> MSFPGWGPYPPVERDETSAITYSSKLHGSVTVRDPYSQLEVPFEDSEETKAFVHSQRKFARTYLDENPDREAWLETLKKSWNYRRFSALKPESDGHYYFEYNDGLQSQLSLYRVRMGEEDTVLTESGPGGELFFNPNLLSLDGNAALTGFVMSP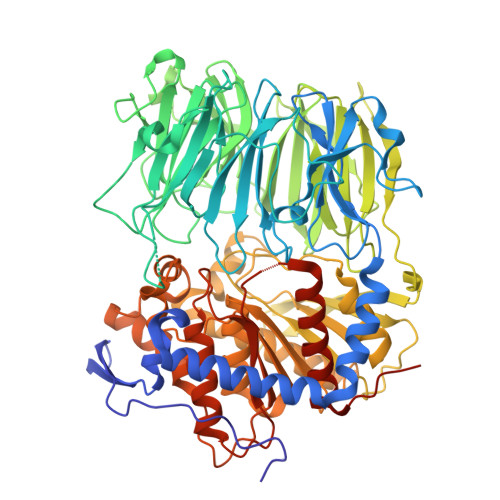CGNYWAYGVSEHGSDWMSIYVRKTSSPHLPSQERGKDPGRMNDKIRHVRFFIVSWTSDSKGFFYSRYPPEDDEGKGNAPAMNCMVYYHRIGEDQESDVLVHEDPEHPFWISSVQLTPSGRYILFAASRDASHTQLVKIADLHENDIGTNMKWKNLHDPWEARFTIVGDEGSKIYFMTNLKAKNYKVATFDANHPDEGLTTLIAEDPNAFLVSASIHAQDKLLLVYLRNASHEIHIRDLTTGKPLGRIFEDLLGQFMVSGRRQDNDIFVLFSSFLSPGTVYRYTFGEEKGYRSLFRAISIPGLNLDDFMTESVFYPSKDGTSVHMFITRPKDVLLDGTSPVLQYGYGGFSLAMLPTFSLSTLLFCKIYRAIYAIPNIRGGSEYGESWHREGMLDKKQNVFDDFNAATEWLIANKYASKDRIAIRGGANGGVLTTACANQAPGLYRCVITIEGIIDMLRFPKFTFGASWRSEYGDPEDPEDFDFIFKYSPYHNIPPPGDTVMPAMLFFTAAYDDRVSPLHTFKHVAALQHNFPKGPNPCLMRIDLNSGHFAGKSTQEMLEETADEYSFIGKSMGLTMQTQGSVDSSRWSCVTV> QFRHLPMPFHWKQEELKFKTGLRRLQHRVGEIHLLREALQKGAEAGQVSLHSLIETPANGTGPSEALAMLLQETTGELEAAKALVLKRIQIWKRQQQLAGNGAPFEESLAPLQERCESLVDIYSQLQQEVGAAGGELEPKTRASLTGRLDEVLRTLVTSCFLVEKQPPQVLKTQTKFQAGVRFLLGLRFLGAPAKPPLVRADMVTEKQARELSVPQGPGAGAESTGEIINNTVPLENSIPGNCCSALFKNLLLKKIKRCERKGTESVTEEK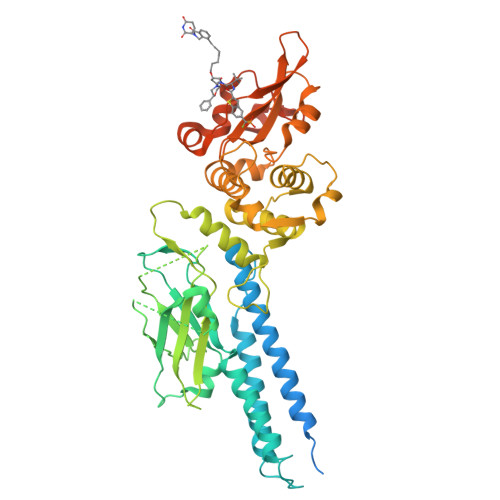CAVLFSASFTLGPGKLPIQLQALSLPLVVIVHGNQDNNAKATILWDNAFSEMDRVPFVVAERVPWEKMCETLNLKFMAEVGTNRGLLPEHFLFLAQKIFNDNSLSMEAFQHRSVSWSQFNKEILLGRGFTFWQWFDGVLDLTKRCLRSYWSDRLIIGFISKQYVTSLLLNEPDGTFLLRFSDSEIGGITIAHVIRGQDGSPQIENIQPFSAKDLSIRSLGDRIRDLAQLKNLYPKKPKDEAFRSHYKPEQMGKDGRGYVPATIKMTVERDQPLPT> IGMAPGGYVA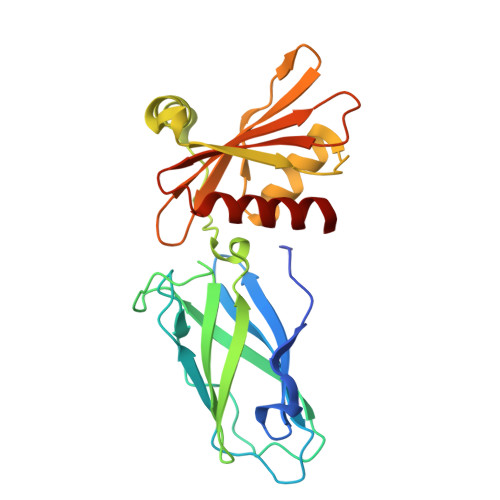PKAVWLPAVKAKGLEISGTFTHRQGHIYMEMNFTNKALQHMTDFAIQFNKNSFGVIPSTPLAIHTPLMPNQSIDVSLPLNTLGPVMKMEPLNNLQVAVKNNIDVFYFSCLIPLNVLFVEDGKMERQVFLATWKDIPNENELQFQIKECHLNADTVSSKLQNNNVYTIAKRNVEGQDMLYQSLKLTNGIWILAELRIQPGNPNYTLSLKCRAPEVSQYIYQVYDSILKN>[2x]MSQEELRQQIAELVAQYAETAMAPKPFEAGKSVVPPSGKVIGTKELQLMVEASLDGWLTTGRFNDAFEKKLGEYLGVPYVLTTTSGSSANLLALTALTSPKLGVRALKPGDEVITVAAGFPTTVNPTIQNGLIPVFVDVDIPTYNVNASLIEAAVSDKTKAIMIAHTLGNLFDLAEVRRVADKYNLWLIEDCCDALGSTYDGKMAGTFGDIGTVSFYPAHHIT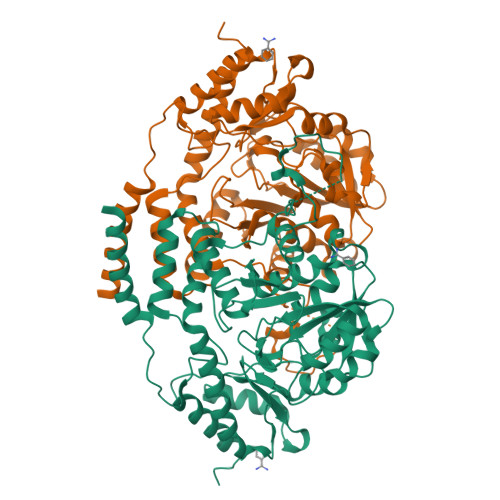MGEGGAVFTQSAELKSIIESFRDWGRDCYCAPGCDNTCKKRFGQQLGSLPFGYDHKYTYSHLGYNLKITDMQAACGLAQLERIEEFVEKRKANFKYLKDALQSCADFIELPEATENSDPSWFGFPITLKEDSGVSRIDLVKFLDEAKVGTRLLFAGNLTRQPYFHDVKYRVVGELTNTDRIMNQTFWIGIYPGLTHDHLDYVVSKFEEFFGLNF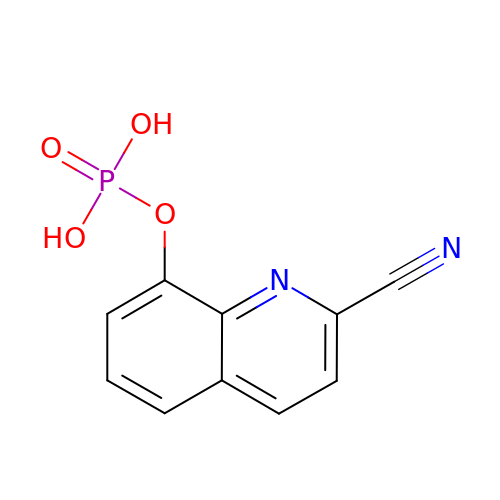2-CYANOQUINOLIN-8-YL DIHYDROGEN PHOSPHATE | C10 H7 N2 O4 P | NQLPTOOPFMPCHQ-UHFFFAOYSA-N> SAYPITGKLGSELTMTDTVGQVVLGWKVSDLKSSTAV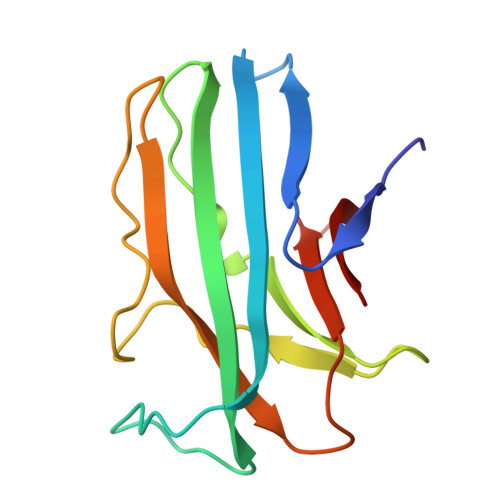IPGYPVAGQVWEATATVNAIRGSVTPAVSQFNARTADGINYRVLWQAAGPDTISGATIPQGEQSTGKIYFDVTGPSPTIVAMNNGMEDLLIWEP> HHHHHHHHHHYDDGICKSSDCIKSAARLIQNMDATTEPCTDFFKYACGGWLKRNVIPETSSRYGNFDILRDELEVVLKDVLQEPKTEDIVAVQKAKALYRSCINESAIDSRGGEPLLKLLPDIYGWPVATENWEQKYGASWTAEKAIAQLNSKYGKKVLINLFVGTDDKNSVNHVIHIDQPRLGLPSRDYYECTGIYKEACTAYVDFMISVARLIRQEERLPIDENQLALEMNKVMELEKEIANATAKPEDRNDPMLLYNKMTLAQIQNNFSLEINGKPFSWLNFTNEIMSTVNISITNEEDVVVYAPEYLTKLKPILTKYSARDLQNLMSWRFIMDLVSSLSRTYKESRNAFRKALYVTTSETATWRRCANYVNGNMENAVGRLYVEAAFAGESKHVVEDLIAQIREVFIQTLDDLTWMDAETKKRAEEKALAIKERIGYPDDIVSNDNKLNNEYLELNYKEDEYFENIIQNLKFSQSKQLKKLREKVDKDEWISGAAVVNAFYSSGRNQIVFPAGILQPPFFSAQQSNS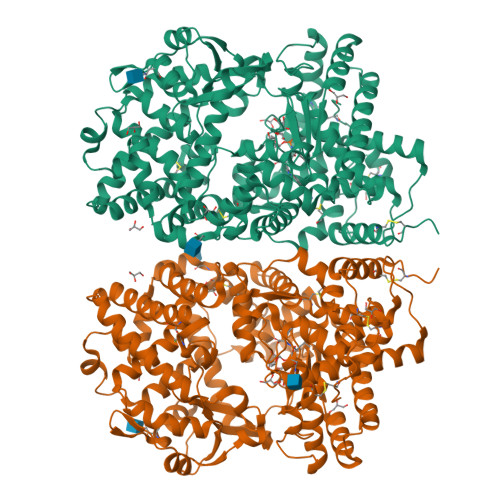LNYGGIGMVIGHEITHGFDDNGRNFNKDGDLVDWWTQQSASNFKEQSQCMVYQYGNFSWDLAGGQHLNGINTLGENIADNGGLGQAYRAYQNYIKKNGEEKLLPGLDLNHKQLFFLNFAQVWCGTYRPEYAVNSIKTDVHSPKNFRIIGTLQNSAEFSEAFHCRKNSYMNPEKKCRVW> MHHHHHHAVRASEISRVYEAYPEKKATLYFLVLGFLALIVGSLFGPFQALNYGNVDAYPLLKRLLPFVQSYYQGLTLHGVLNAIVFTQLFAQAIMVYLPARELNMRPNMGLMWLSWWMAFIGLVVAALPLLANEATVLYTFYPPLKGHWAFYLGASVFVLSTWVSIYIVLDLWRRWKAANPGKVTPLVTYMAVVFWLMWFLASLGLVLEFVLFLLPWSFGLVEGVDPLVARTLFWWTGHPIVYFWLLPAYAIIYTILPKQAGGKLVSDPMARLAFLLFLLLSTPVGFHHQFADPGIDPTWKMIHSVLTLFVAVPSLMTAFTVAASLEFAGRLRGGRGLFGWIRALPWDNPAFVAPVLGLLGFIPGGAGGIVNASFTLDYVVHNTAWVPGHFHLQVASLVTL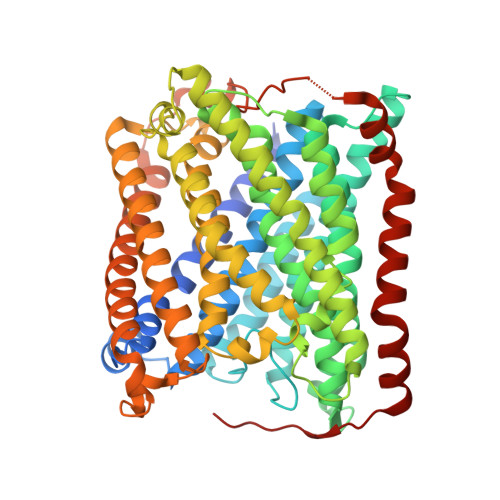TAMGSLYWLLPNLTGKPISDAQRRLGLAVVWLWFLGMMIMAVGLHWAGLLNVPRRAYIAQVPDAYPHAAVPMVFNVLAGIVLLVALLLFIYGLFSVLLSRERKPELAEAPLPFAEVISGPEDRRLVLAMDRIGFWFAVAAILVVLAYGPTLVQLFGHLNPVPGWRLW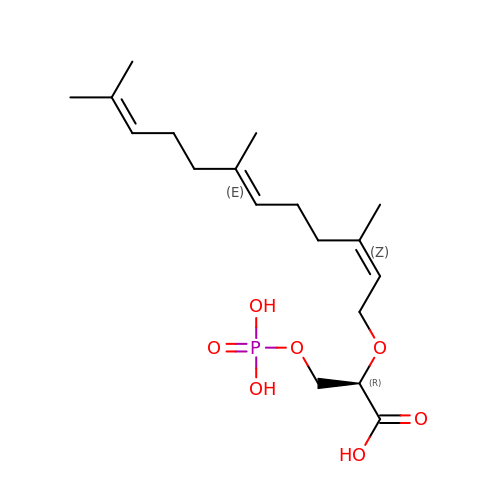(2R)-3-(phosphonooxy)-2-{[(2Z,6E)-3,7,11-trimethyldodeca-2,6,10-trien-1-yl]oxy}propanoic acid | C18 H31 O7 P | SLQQIKXGDCLCGX-XLGHFPRDSA-N>AGHSGRAKAVARLSDLLSTDPLGRLTEVEELLRAHAPTAADFARLFEACAERLTRALAEDRISRMQVTLAYSAL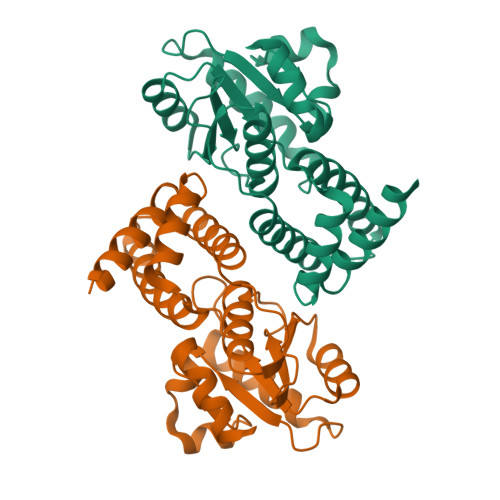QMALRRIHHLPDPQKSVGAVLVAGVPGHKPILEAALAAEMLRAVGWSTSVVHPESVAALAARLKTSRTSTLVVAPSLLEGTEQEADTLRFVSALRARTDLPGLSILVGGRLAQLPPSKLKDSGADAGFAHLALLPAALARVA[2x]>[4x]DSDDRVTPPAEPLDRMPDPYRPSYGRAETVVNNYIRKWQQVYSHRDGRKQQMTEEQREWLSYGCVGVTWVNSGQYPTNRLAFASFDEDRFKNELKNGRPRSGETRAEFEG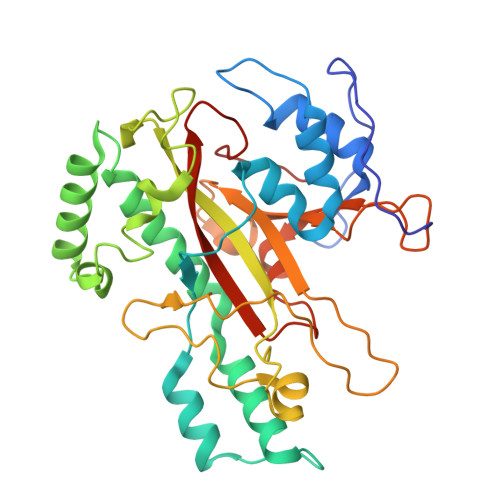RVAKESFDEEKGFQRAREVASVMNRALENAHDESAYLDNLKKELANGNDALRNEDARSPFYSALRNTPSFKERNGGNHDPSRMKAVIYSKHFWSGQDRSSSADKRKYGDPDAFRPAPGTGLVDMSRDRNIPRSPTSPGEGFVNFDYGWFGAQTEADADKTVWTHGNHYHAPNGSLGAMHVYESKFRNWSEGYSDFDRGAYVITFIPKSWNTAPDKVKQGWP> TVTVTYDPSNAPSFQQEIANAAQIWNSSVRNVQLRAGGNADFSYYEGNDSRGSYAQTDGHGRGYIFLDYQQNQQYDSTRVTAHETGHVLGLPDHYQGPCSELMSGGGPGPSCTNPYPNAQERSRVNALWA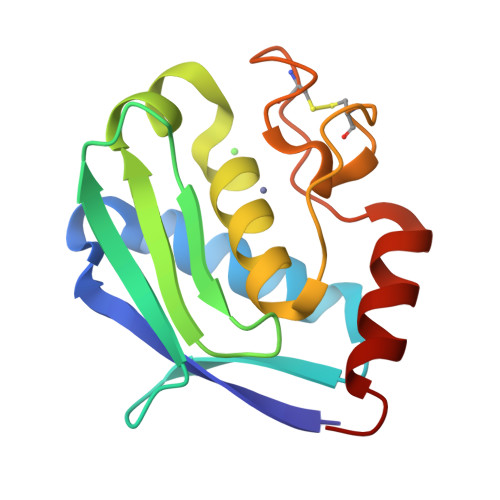NG> KIPVDADFLYAYSTAPGYYSWRNSK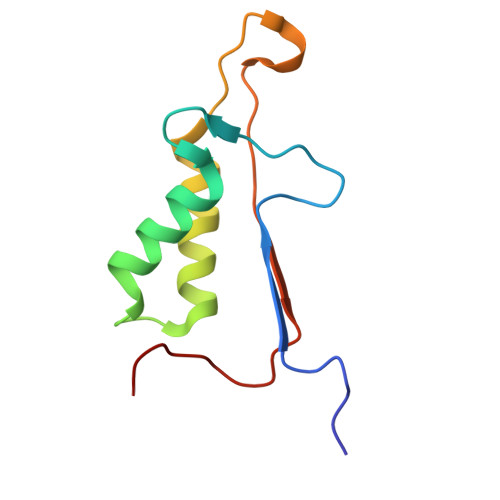DGSWFIQSLCAMLKQYADKLEFMHILTRVNRKVATEFESFSFDATFHAKKQIPCIVSMLTKELYFYH>[6x]MQTKKNEIWVGIFLLAALLAALFVCLKAANVTSIRTEPTYTLYATFDNIGGLKARSPVSIGGVVVGRVADITLDPKTYLPRVTLEIEQRYNHIPDTSSLSIRTSGLLGEQYLALNVGFEDPELGTAILKDGDTIQDTKSAMVLEDLIGQFLYGSKGDDNKNSGDAPAAAPGNNETTEPVGTTK;>[2x]MSESLSWMQTGDTLALSGELDQDVL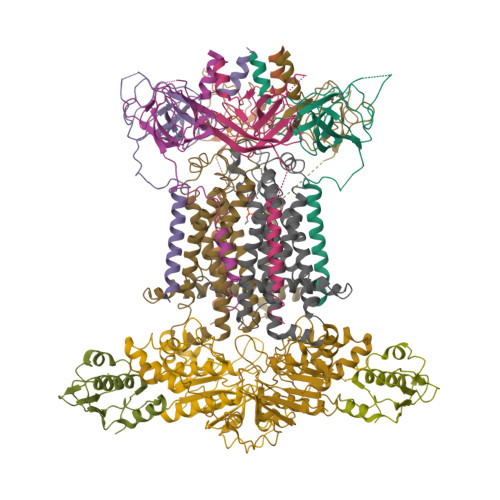LPLWEMREEAVKGITCIDLSRVSRVDTGGLALLLHLIDLAKKQGNNVTLQGVNDKVYTLAKLYNLPADVLPRHHHHHHHH;>[2x]MLLNALASLGHKGIKTLRTFGRAGLMLFNALVGKPEFRKHAPLLVRQLYNVGVLSMLIIVVSGVFIGMVLGLQGYLVLTTYSAETSLGMLVALSLLRELGPVVAALLFAGRAGSALTAEIGLMRATEQLSSMEMMAVDPLRRVISPRFWAGVISLPLLTVIFVAVGIWGGSLVGVSWKGIDSGFFWSAMQNAVDWRMDLVNCLIKSVVFAITVTWISLFNGYDAIPTSAGISRATTRTVVHSSLAVLGLDFVLTALMFGN;>[2x]MEQSVANLVDMRDVSFTRGNRCIFDNISLTVPRGKITAIMGPSGIGKTTLLRLIGGQIAPDHGEILFDGENIPAMSRSRLYTVRKRMSMLFQSGALFTDMNVFDNVAYPLREHTQLPAPLLHSTVMMKLEAVGLRGAAKLMPSELSGGMARRAALARAIALEPDLIMFDEPFVGQDPITMGVLVKLISELNSALGVTCVVVSHDVPEVLSIADHAWILADKKIVAHGSAQALQANPDPRVRQFLDGIADGPVPFRYPAGDYHADLLPGS In order to decipher the structural basis of their substrate specificities and to provide a rational, we structurally and biochemically characterized two 1β aminotransferases from Mycobacterium tuberculosis (Mtb), an HspAT, encoded by rv1600 (mHspAT) and a putative phenylalanine aminotransferase, encoded by rv3772. However, experimental characterisation of this aminotransferase in the current study clearly demonstrates high catalytic preference for Phe, Tyr and Trp instead for Hsp. Therefore, we propose its reannotation of as an aromatic amino acid aminotransferase (mArAT). Contrastingly in mArAT, residues Val86, Phe110, Leu112 and Phe246* form a hydrophobic substrate binding pocket which provides an energetically favourable environment for the specific binding of hydrophobic substrates such as Phe, Trp and the less polar Tyr.

We also report the experimentally determined structure of mArAT-aromatic amino acid complex. The binding of Phe and succinate in the active site of mArAT as observed in the crystal structures of mArAT-PLP-Phe and mArAT-PMP-succinate complexes revealed the molecular basis of substrate selectivity of mArAT. The two liganded structures are virtually identical (an rmsd of 0.28 Å over 305 Cα atom pairs). In the substrate bound mArAT complex, Phe is present in the active site of both the monomers of a homodimer, though it exists as a PLP-Phe external aldimine intermediate complex in one of the monomers, and as free-Phe in the other monomer. The carboxylate group of free-form of Phe is held in place through interactions with Asn157 and the PLP bound-form makes an additional interaction with Arg330. The N-terminal lid regulates the entry and binding of Phe by rearranging the side chains of Tyr15, along with Glu111, Leu112 and Arg322. A stretch of residues of the lid exhibit plasticity (Leu9 to Ala24, rmsd 2.9 Å over 16 aligned Cα pairs), by adopting different conformations in free- and Phe bound form. Tyr15 forms a H-bond with Arg322 when Phe is covalently linked to the cofactor in one monomer. In the other monomer, the carboxylate group of ‘free’ Phe form H-bond with Arg322. The present structures clearly demonstrate the role of the “arginine switch” mechanism in the binding of the carboxylate group of Phe in which Arg322 moves away from the active site to allow the access of the bulky head group of Phe.

>MVTARLRPELAGLPVYVPGKTVPGAIKLASNETVFGPLPSVRAAIDRATDTVNRYPDNGCVQLKAALARHLGPDFAPEHVAVGCGSVSLCQQLVQVTASVGDEVVFGWRSFELYPPQVRVAGAIPIQVPLTDHTFDLYAMLATVTDRTRLIFVCNPNNPTSTVVGPDALARFVEAVPAHILIAIDEAYVEYIRDGMRPDSLGLVRAHNNVVVLRTFSKAYGLAGLRIGYAIGHPDVITALDKVYVPFTVSSIGQAAAIASLDAADELLARTDTVVAERARVSAELRAAGFTLPPSQANFVWLPLGSRTQDFVEQAADARIVVRPYGTDGVRVTVAAPEENDAFLRFARRWRSDQKLAAALEHHHHHH[4x]> MWSHPQFEKENLYFQGSMDDISPSELKTILHSKRANLYYLQHCRVLVNGGRVEYVTDEGRHSHYWNIPIANTTSLLLGTGTSITQAAMRELARAGVLVGFCGGGGTPLFSANEVDVEVSWLTPQSEYRPTEYLQRWVGFWFDEEKRLVAARHFQRARLERIRHSWLEDRVLRDAGFAVDATALAVAVEDSARALEQAPNHEHLLTEEARLSKRLFKLAAQATRYGEFVRAKRGSGGDPANRFLDHGNYLAYGLAATATWVLG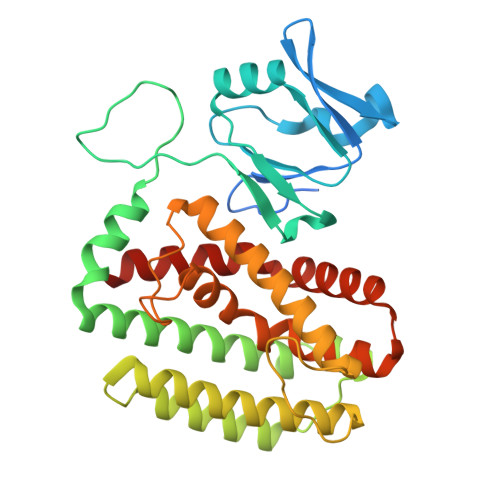IPHGLAVLHGKTRRGGLVFDVADLIKDSLILPQAFLSAMRGDEEQDFRQACLDNLSRAQALDFMIDTLKDVAQRSTVSA> MRYIRLCIISLLATLPLAVHASPQPLEQIKLSESQLSGRVG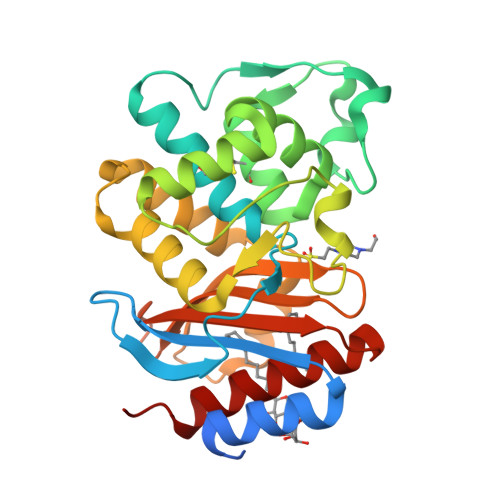MIEMDLASGRTLTAWRADERFPMMSTFKVVLCGAVLARVDAGDEQLERKIHYRQQDLVDYSPVSEKHLADGMTVGELCAAAITMSDNSAANLLLATVGGPAGLTAFLRQIGDNVTRLDSWETELNEALPGDARDTTTPASMAATLRKLLTSQRLSARSQRQLLQWMVDDRVAGPLIRSVLPAGWFIADKTGAGERGARGIVALLGPNNKAERIVVIYLRDTPASMAERNQQIAGIGAALIEHWQR>[2x]MQTLSERLKKRRIALKMTQTELATKAGVKQQSIQLIEAGVTKRPRFLFEIA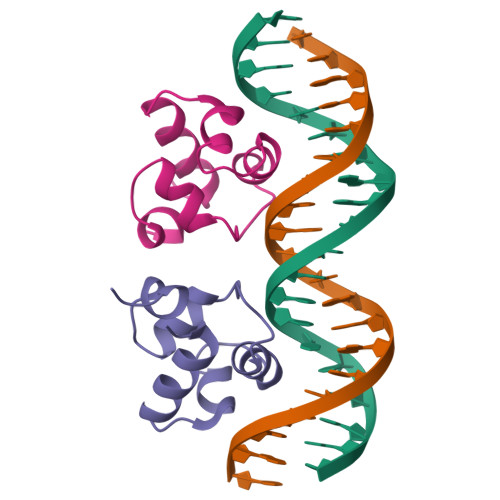MALNCDPVWLQYGTKRGKAA> RRRRWRER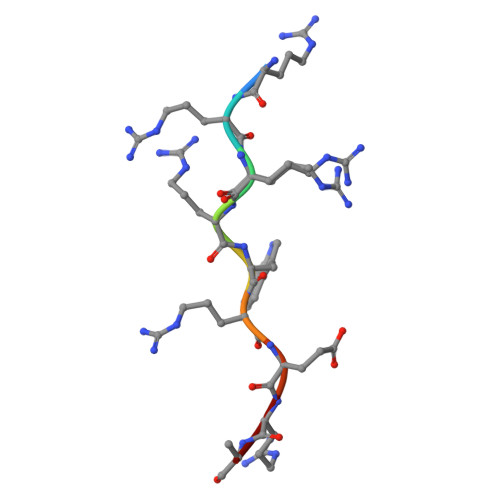Q> GSSQAKPPTRLFRGLNLSEEFTKGLIDQANAMIANTTERLFTDHSPEAFKQIKLNDLSKMSGRTNASTTTEIKLVKETWDSNVIFEMLDPDGLLHSKQVGRHGEGTASAFSVYLPEDVALVPV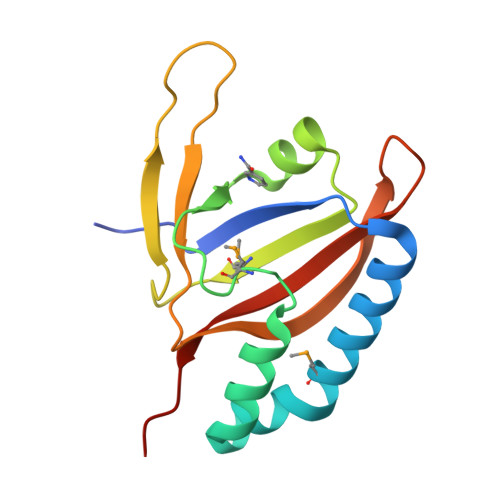KVTLDGKTQKGENRYVFTFVAVKSPDFTP> MATATEQWVLVEMVQAL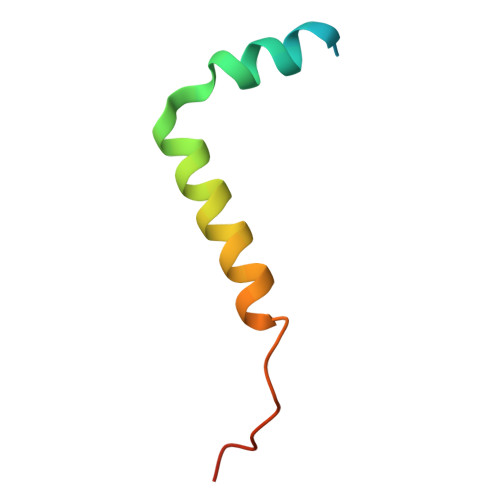YEAPAYHLILEGILILWIIRLLFSKTYKLQERS> GIEY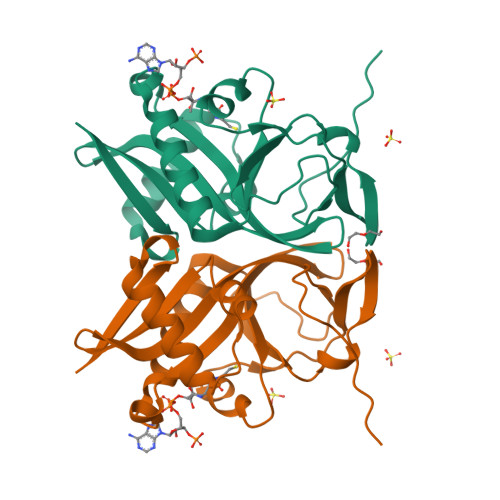RSLHTSQLTLSEKEALYDLLIEGFEGDFSHDDFAHTLGGMHVMAFDQQKLVGHVAIIQRHMALDNTPISVGYVEAMVVEQSYRRQGIGRQLMLQTNKIIASCYQLGLLSASDDGQKLYHSVGWQIWKGKLFELKQGSYIRSIEEEGGVMGWKADGEVDFTASLYCDFRGGDQWLEHHH>GAMAVIDNSTKTLEQQTAQTNVAALPAITVKAEQDDTYAGGQVATSSNVGFLGSKKFLDTPFNTISYTDKYIEDKQAKDITEVIAATDPSIYTNGASGGWSENYYIRGYASSTNDMSMNGLFGITPFYRTSPEMFGRVEVLKGPSALLNGMPPAGSVGGTVNLVTKYAADEPFARLTTTYMSDAQFGGHVDVGRRFGENKEFGVRINGMYRDGDAAVNDQSKESRLFSLGLDWQGENARVFVDAYDALDHVDGVTRGVNVSTAVGIPKPPKADTLLSP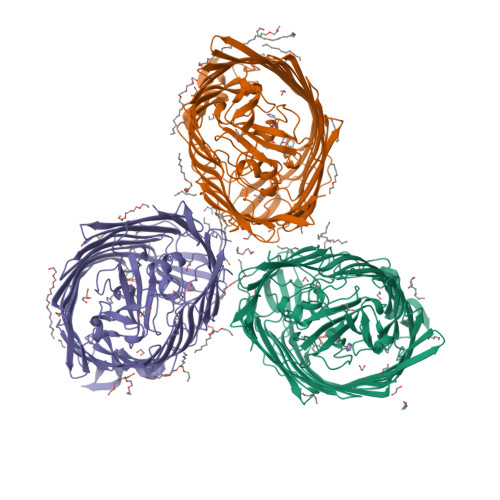DWGSVETKDKGAMIRGEYDFSDQLMAYAAYGQSTTEYKYNGASAGTITSSTGTLSSTLGQLAFDVDKKSADAGFKGKFETGSVKHQWVANATYYNHTQDDYGYRIIPGFSDPVITNIYDPNPNWGPKPEFTPPFLFHSTLSTSSFGLADTLSFAQDKVQLTLGLRHQTVKATSSVNTLPENAKSATTPGVALLIKATDKISVYANYIEGLTKGDQAPATASNPGEIFPPQKTKQQELGLKVDLGTFAHTLSAFEITKPSSYLDPSKLVNNLPTFVSDGEQRNRGIEWSFFGSPIEHVRLMGGFTYLDPELTKTKSGGNDGHTAVAVPKNQAKLGAEWDTQVAQGTLTLSGNINAVSKQYINAENTLSVPGRTLLDVGARYSTKVEDHPVTFRANIYNLTNKAYWAQPQLTNLALGAPRTYMLSVSYDF[3x]> MREYKLVVLGSGGVGKSA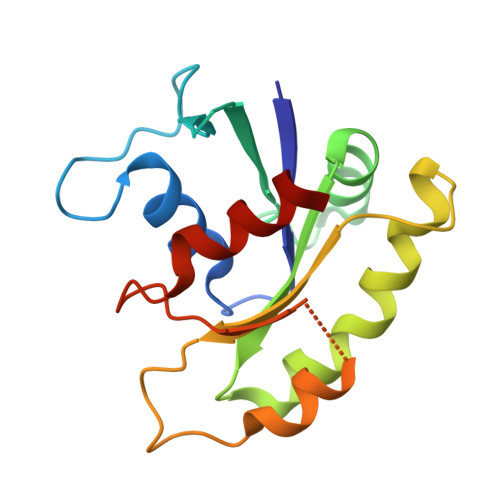LTVQFVQGIFVEKYDPTIEDSYRKQVEVDAQQCMLEILDTAGTEQFTAMRDLYMKNGQGFALVYSITAQSTFNDLQDLREQILRVKDTDDVPMILVGNKCDLEDERVVGKEQGQNLARQWNNCAFLESSAKSKINVNEIFYDLVRQINR> GARDVQEGVSSFEESGGAQLPPRVHALEVLEGAGPGRLHGRLGIKPDGQPGYTRAPSPPTDLSMPQALARGGGFNLYLSDHLELDRTAPDARHASCRQLHYDLSTLPKASVIIVFYNEPFSTLMRSVHSVLNGTPPQILEELILVDDGSTLPYIREDGNQQLVEYLKLLPAKVRLIRNEVRKGIVGARMKGIRASRAPIFAILDSHIEVSPQWLEPLLLRIKEDSRRVVMPQIDGIDAETFKHIAGGIGCKLGFLWKLMEHSYEGHQTARLPPEERQPSPTDFQTSPAMAGGLFAANKAFFFDVGAYDEDFQFWGTENLELSFRLWQCGGVLECAPCSRVYHIFRKGGSGYSSPGDSITINKMRTMLWMDEYADLAWRVIGKPRVNYRPESLEKRREWRKRKGCKSFRWFMENVFPEGDVVTLDDVPYLGPLRNDKIGMCLDNMGWASPGHAVGLEYCHGGDTQTFMFFRKVGHVMPVNDDEACLQPSGRLDWCRGTAQFWWDFTSSGQLMFRETKQCLSAFGRKLRMVECDDTDPYQIWSWTAYNPPDTFTFPSVSRSIRSG;> GTTPSPVPTTSTTSAP

O-glycosylation of the protein CST1 by the mucin-type O-glycosyltransferase T. gondii (Txg) GalNAc-T3 influences cyst wall rigidity and stability. The strict glycopeptide-preferring enzyme TxgGalNAc-T3 then adds GalNAc to acceptor Thr one position N-terminal to existing Thr-O-GalNAcs and is predicted to sequentially O-glycosylate Thr rich repeats within the mucin domain of CST1. The structures reveal a unique GalNAc binding pocket that dictates the substrate preference of TxgGalNAc-T3, which is coupled to a 2nd metal binding site that is strictly conserved among apicomplexan homologs.

To investigate the basis of the substrate specificity and function of TxgGalNAc-T3, we solved the x-ray co-crystal structures of TxgGalNAc-T3 in complex with Mn2+, a non-hydrolysable form of UDP-GalNAc (UDP-2-(acetylamino)−4-F-D-galactosamine disodium salt, UDP-GalNAc-F) and each of the following glycopeptides: CST1.4, Muc5AC-3,13, Muc5AC-3, Muc5AC-13, and SRS13.2 from 2.2-2.9 Å resolution. Although the glycopeptide amino acid sequences vary, both CST1.4 and Muc5AC-3,13 are similarly bound along the active site substrate groove with the acceptor Thr positioned for catalysis, adopting a similar conformation seen in peptides bound to metazoan GalNAc-Ts. Poor electron density for the remaining unmodeled residues in CST1.4 and Muc5AC-3,13 suggests that they are disordered in the structure and making transient interactions with TxgGalNAc-T3. We could not model the peptide substrate in the structure containing Muc5AC-13 due to unresolvable electron density, and we only observe weak density for Thr-O-GalNAc in the SRS13.2 structure. It is notable that the di-glycopeptides were the only substrates with electron density for the N-terminal portion of the peptide chain, but it is not clear what is stabilizing the peptide conformations in these structures since we did not observe density for the C-terminal residues. Thr-O-GalNAc at the +1 position on the glycopeptides is bound to a pocket in TxgGalNAc-T3 consisting of His333 (catalytic domain) and Glu554 (lectin domain) that interact with GalNAc via sidechain H-bonds, and Ser334 (catalytic domain), which interacts with GalNAc through a mainchain H-bond. We observed density that appears to be a 2nd metal (Mn2+N) near the GalNAc binding pocket, a striking and unexpected feature not previously seen in metazoan GalNAc-Ts. Mn2+N is coupled to the GalNAc binding pocket through coordination to His333 and indirect coordination to Glu554 via water. Glu336 and 2 additional waters complete the coordination sphere of Mn2+N, which adopts an irregular octahedral geometry. Loop II flexibility and the interaction that occurs between the Gly319 backbone carbonyl and an amide group on both di-glycopeptide substrates (Muc5AC-3,13 and CST1.4) allows TxgGalNAc-T3 to accommodate and modify substrates with variable sequences.TMEM120A, also named as TACAN, is a novel membrane protein highly conserved in vertebrates and was recently proposed to be a mechanosensitive channel involved in sensing mechanical pain. Here we present the single-particle cryogenic electron microscopy (cryo-EM) structure of human TMEM120A, which forms a tightly packed dimer with extensive interactions mediated by the N-terminal coiled coil domain (CCD), the C-terminal transmembrane domain (TMD), and the re-entrant loop between the two domains. The TMD of each TMEM120A subunit contains six transmembrane helices (TMs) and has no clear structural feature of a channel protein. Intriguingly, some structural features of TMEM120A resemble those of elongase for very long-chain fatty acids (ELOVL) despite the low sequence homology between them, pointing to the possibility that TMEM120A may function as an enzyme for fatty acid metabolism, rather than a mechanosensitive channel.

Human TMEM120A was expressed in HEK293F cells using the BacMam system, solubilized in lauryl maltose neopentyl glycol (LMNG) detergent, and finally purified in digitonin detergent as a homo-dimer ('Materials and methods'). The single-particle cryo-EM structure of TMEM120A dimer was determined to the resolution of 3.2 Å (Figure 2—figure supplements 1–3, and Figure 2—source data 1). The EM density map is of high quality, allowing for accurate model building for the major part of the protein containing residues 8–69, 80–255, and 261–335 for each subunit. Dimerization starts at CCD where the exceptionally long (~60 residues) CC1 helix forms an anti-parallel coiled coil with CC1 from the neighboring subunit. The re-entrant loop of each subunit is tightly wedged between the two TMDs of the dimer at the internal leaflet of the membrane. It mediates another set of extensive dimerization interactions through predominantly Van der Waals contacts with the re-entrant loop from the neighboring subunit as well as the internal halves of TMDs from both subunits. This insertion of the re-entrant loops between the two subunits splits apart the two TMDs at the internal leaflet of the membrane and consequently the two TMDs make direct contact only at the external leaflet of the membrane through some hydrophobic residues at the external parts of TM2, TM3, and TM6, rendering the TMEM120A dimer with an arrowhead-shaped transmembrane region. The transmembrane α-helical barrel enclosed a deep pocket only open to the inside but completely sealed off from the outside. Thus, no discernible ion conduction pathway is present in the TMD of TMEM120A. In TMEM120A structure, we also observed a piece of well-resolved electron density in the pocket of the 6-TM barrel that fits well with a CoA molecule. Despite the low sequence homology, the 6-TM barrel structure of ELOVL7 is strikingly similar to that of TMEM120A (TMs 1–6) with a main-chain RMSD of about 2.5 Å between their barrel-forming 6-TM helices.

>[2x]MDYKDDDDKGGSASQPPPPGPLGDCLRDWEDLQQDFQNIQETHRLYRLKLEELTKLQNNCTSSITRQKKRLQELALALKKCKPSLPAEAEGAAQELENQMKERQGLFFDMEAYLPKKNGLYLSLVLGNVNVTLLSKQAKFAYKDEYEKFKLYLTIILILISFTCRFLLNSRVTDAAFNFLLVWYYCTLTIRESILINNGSRIKGWWVFHHYVSTFLSGVMLTWPDGLMYQKFRNQFLSFSMYQSFVQFLQYYYQSGCLYRLRALGERHTMDLTVEGFQSWMWRGLTFLLPFLFFGHFWQLFNALTLFNLAQDPQCKEWQVLMCGFPFLLLFLGNFFTTLRVVHHKFHSQRHGSKKD>[5x]TPQN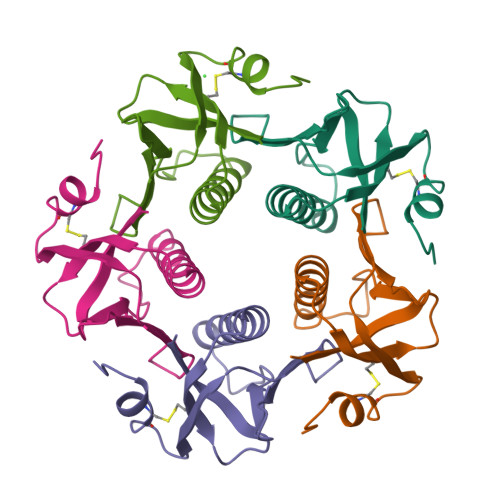ITDLCAEYHNTQIHTLNDKIFSYTESLADKREMAIITFKNGATFQVEVPGSQHIDSQKKAIERMKDTLRIAYLTEAKVEKLCVWNNKTPHAIAAISMAN> GAGCAGACATGA;> CGTCACTCA;> TCAACG;> TCTGAGTGTGTCTG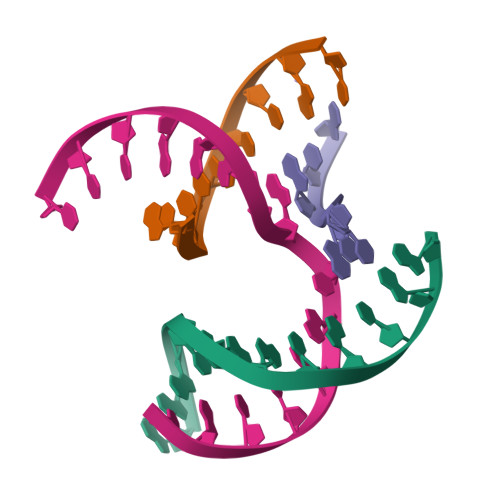C>[2x]AAGVDNYVIQYLKV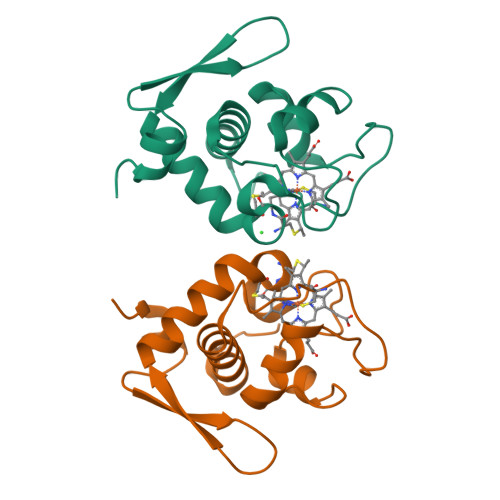TDTVELPVNDRGETKTFTAVDLTRGKRLFEENCKNCHVGGSTLPNPLVSLSLKDLKGATPPRDTIASLVAFQRSPKSYDGSEESYSCRRVSEDWLTTEQLETLAAFILRAAAVAPGWGVESFPDSAP>MSLSDQSQIIAGFTLWHLSLPVTARRDHGIGSVAGAVEVVVLRLQADSGAVGYGEASPWVVFTGSVEATYAALDRYLRPLVLGRAVGDHAAIMEDARAAVAHCTEAKAALDTALYDLRARIAGVPVWALLGGRCRDRIPLSCSIADPDFDKDLALMQRLQDDDVRIIKLKTGFKDHAFDMMRLERLRADFPAFDIRVDYNQGLHH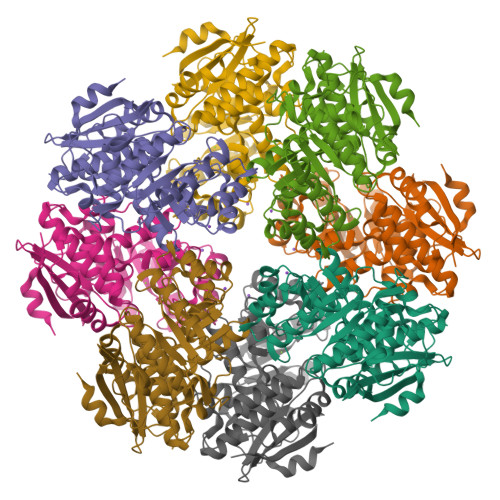DVALARVRDVATFKPTFIEQPVKAHLRGLMARIRDAVDVPLLADESIFGPEDMAEHPEIADGVSIKIMKSGGLTRAQTVARMAAARGLSAYGGDMFEAGLAHLAGAHMIAATPEITLGCEFYQATYFLCDDILAAPFPVADGHVLVPDTPGLGVDVDEDALARFAVAREGHHHHHH[4x]> MSTSSLRRQMKNIVHNYSEAEIKVREATSNDPWGPSSSLMSEIADLTYNVVAFSEIMSMIWKRLNDHGKNWRHVYKAMTLMEYLIKTGSERVSQQCKENMYAVQTLKDFQYVDRDGKDQGVNVREKAKQLVALLRDEDRLRE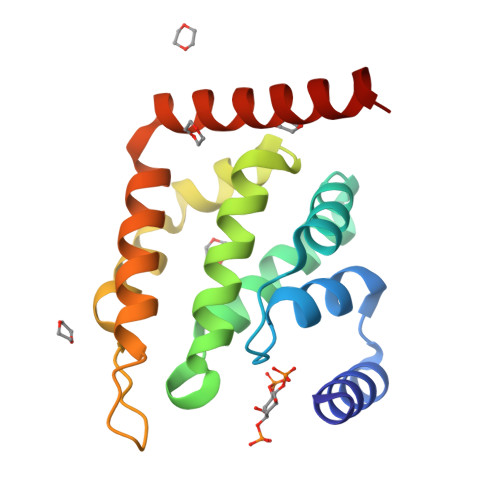ERAHALKTKEKLAQTA N-((1R,2S,5S)-2-(5-CHLORO-1H-INDOLE-2-CARBOXAMIDO)-5-(DIMETHYLCARBAMOYL)CYCLOHEXYL)-5-METHYL-4,5,6,7-TETRAHYDROTHIAZOLO[5,4-C]PYRIDINE-2-CARBOXAMIDE | C26 H31 Cl N6 O3 S | 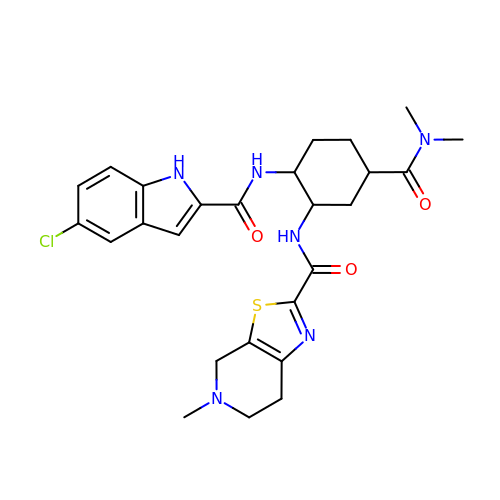SZBHQQIIGORYND-ADLFWFRXSA-N>[2x]MTQPLVGKQILIVEDEQVFRSLLDSWFSSLGATTVLAADGVDALELLGGFTPDLMICDIAMPRMNGLKLLEHIRNRGDQTPVLVISATENMADIAKALRLGVEDVLLKPVKDLNRLREMVFAC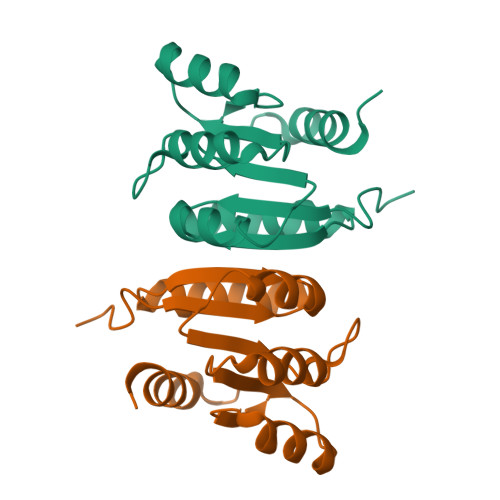LYPSMFNSRVEEEERLFRDWDAMVDNPAAAAKLLQELQPPVQQVISHCRVNYRQLVAADKPGLVLDIAALSENDLAFYCLDVTRAGHNGVLAALLLRALFNGLLQEQLAHQNQRLPELGALLKQVNHLLRQANLPGQFPLLVGYYHRELKNLILVSAGLNATLNTGEHQVQISNGVPLGTLGNAYLNQLSQRCDAWQCQIWGTGGRLRLMLSAE> GPMNIINTSILNLRYESNHLIDLSRYASKINIGSKVNFDPIDKNQIQLFNLESSKIEVILKNAIVYNSMYENFSTSFWIRIPKYFNSISLNNEYTIINCMENNSGWKVSLNYGEIIWTLQDTQEIKQRVVFKYSQMINISDYINRWIFVTITNNRLNNSKIYINGRLIDQKPISNLGNIHASNNIMFKLDGCRDTHRYIWIKYFNLFDKELNEKEIKDLYDNQSNSGILKDFWGDYLQYDKPYYMLNLYDPNKYVDVNNVGIRGYMYLKGPRGSVMTTNIYLNSSLYRGAKFIIKKYASGNKDNIVRNNDRVYINVVVKNKEYRLATNASQAGVEKILSALEIPDVGNLSQV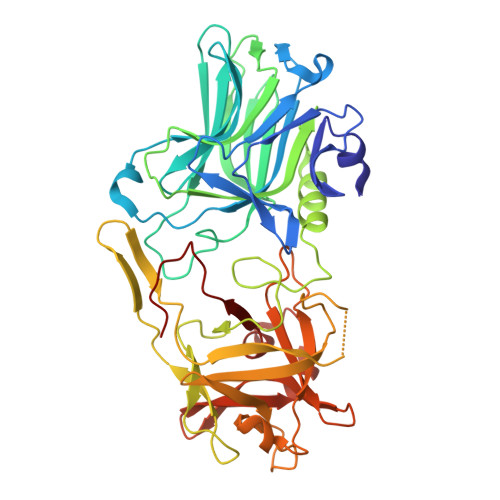VVMKSKNDQGITNKCKMNLQDNNGNDIGFIGFHQFNNIAKLVASNWYNRQIERSSRTLGCSWEFIPVDDGWGERPL3,5-dichloro-L-tyrosine | C9 H9 Cl2 N O3 | 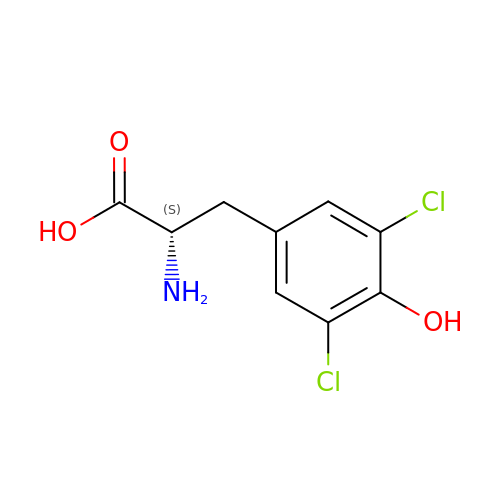MPHURJQUHZHALJ-ZETCQYMHSA-N>[3x]GTTTDDLLTRYRANPAMMKNLKLSDIRGALLKFAKDQVGSRFIQQELASSKDRFEKDSIFDEVVSNADELVDDIFGNYVVQKFFEYGEERHWARLVDAIIDRVPEYAFQMYACRVLQKALEKINEPLQIKILSQIRHVIHRCMKDQNGNHVVQKAIEKVSPQYVQFIVDTLLESSNTIYEMSVDPYGCRVVQRCLEHCSPSQTKPVIGQIHKRFDEIANNQYGNY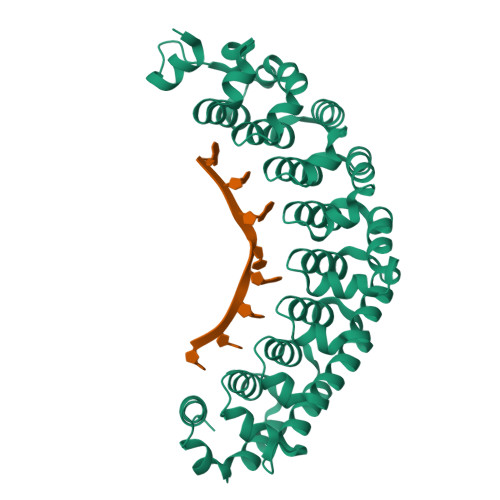VVQHVIEHGSEEDRMVIVTRVSNNLFEFATHKYSSNVIEKCLEQGAVYHKSMIVGAACHHQEGSVPIVVQMMKDQYANYVVQKMFDQVTSEQRRELILTVRPHIPVLRQFPHGKHILAKLEKYFQKPAVMS> HMSELSEIDSVAGVTIYSVDGEPKSFVYKAGFAIDADGAPNAYAPNNGGTDFTANGGDDQGGDWWGGPVDAEGYPIKQKIFDPFPGYYVSATAHFNPAYSEDSPYRYIDSNSIPFIVLPGNHSNGAKLGDVALVYNEKTGDNCYAIYGNVGPSSKIGEGSVRLAQALKIDDNPKAGGTESRIVVTLVFPGSVGKWETPKRWFSHANQLTKAWGGLSRLKTLSDQL

We focus on AMGs that potentially encode chitosanase enzymes that metabolize chitin – a common carbon polymer. One expressed protein showing endo-chitosanase activity (V-Csn) is crystalized and structurally characterized at ultra-high resolution, thus representing the structure of a soil viral AMG product. The structure consisted of two non-contiguous structural domains. Our rigorous analyses not only resulted in a crystal structure of a soil viral AMG product, but also enabled us to propose the mode of action of this previously uncharacterized chitosanase enzyme in the GH75 family of glycosyl hydrolases.

Based upon a partial alignment of the V-Csn, A. fumigatus, F. solani, and S. avermitilis sequences, the corresponding residues in V-Csn are D148 and E157. Two V-Csn constructs harboring either a D148N substitution or a E157Q substitution were generated, and the activities of the respective mutant enzymes measured. Activity was reduced five-fold for D148N and almost eliminated for E157Q. Both constructs eluted with gel-filtration chromatography retention times identical to native V-Csn, and circular dichroism spectra indicated both constructs were folded. In both cases the carboxylate was converted to the corresponding amide, generating the mutant proteins D148N and E157Q. The two mutant V-Csn proteins were crystallized under the same conditions as the wild-type protein, and their structures were determined by molecular replacement to high resolution. Superposition of the two mutant structures onto the wild-type apo1 structure gave RMSDs of 0.11 and 0.07 Å, respectively, for all Cα positions, suggesting very little conformational differences between the mutant and the wild-type structures. Co-crystallization of both mutant proteins with chitohexaose (a β-(1-4)-linked polymer of six D-glucosamine (GlcN) residues) gave a complex with the E157Q mutant only.>FACKTANGTAIPIGGGSANVYVNLAPVVNVGQNLVVDLSTQIFCHNDYPETITDYVTLQRGSAYGGVLSNFSGTVKYSGS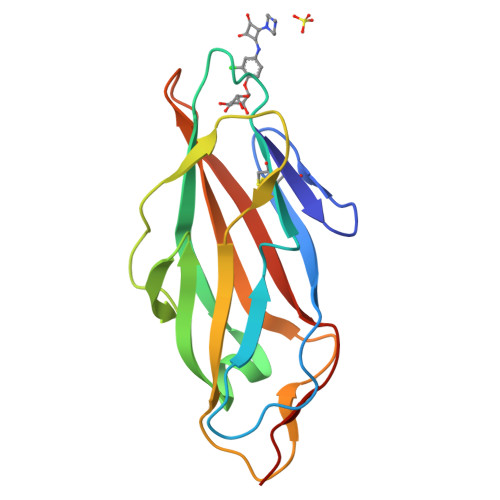SYPFPTTSETPRVVYNSRTDKPWPVALYLTPVSSAGGVAIKAGSLIAVLILRQTNNYNSDDFQFVWNIYANNDVVVPTGL[3x]> MSNPS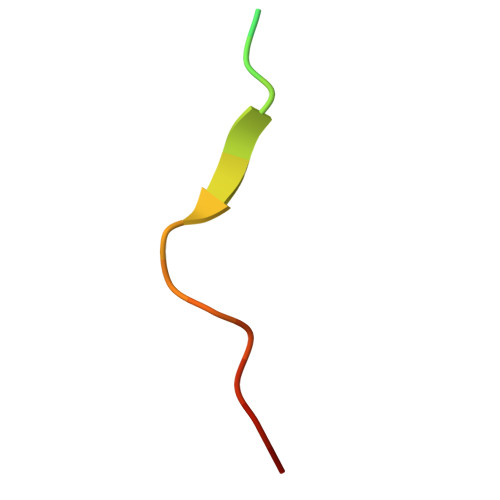ASSGPWKPAKPAPSVS>AMGKCPTKVVLLRNMVGAGEVDEDLEVETKEECEKYGKVGKCVIFEIPGAPDDEAVRIFLEFERVESAIKAVVDLNGRYFGGR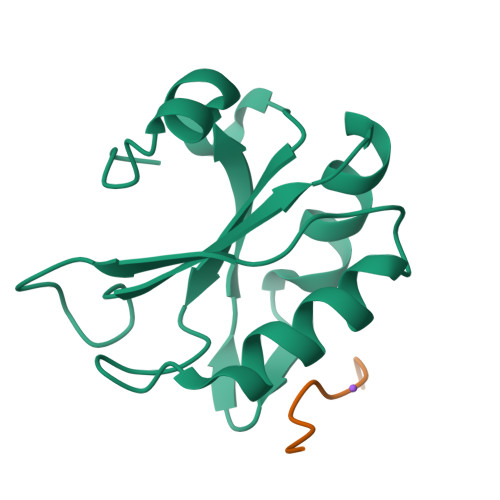VVKACFYNLDKFRVLDLAEQV[2x];> RRRRWRERQ> MGHHHHHHMNAEKSPVNHNVDHEEIAKFEAVASRWWDLEGEFKPLHRINPLRLGYIAERAGGLFGKKVLDVGCGGGILAESMAREGATVTGLDMGFEPLQVAKLHALESGIQVDYVQETVEEHAAKHAGQYDVVTCMEMLEHVPDPQSVVRACAQLVKPGGDVFFSTLNRN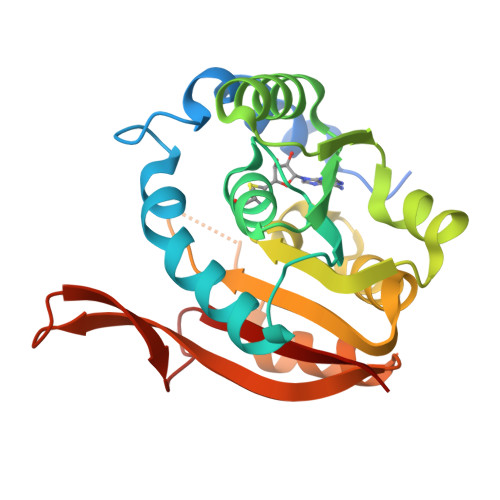GVKKFIKPAELLGWVDQTSLKERHITGLHYNPITNTFKLGPGVDVNYMLHTQNK> MAEVKANGFPGWLLDPLRPTREKAEPRYRLPEDVRIWAVPLAIGVGLLIVSLVGWAIDARQFYFSYLVGWTFCLTLALGSLFFVMIQHLTRAQWV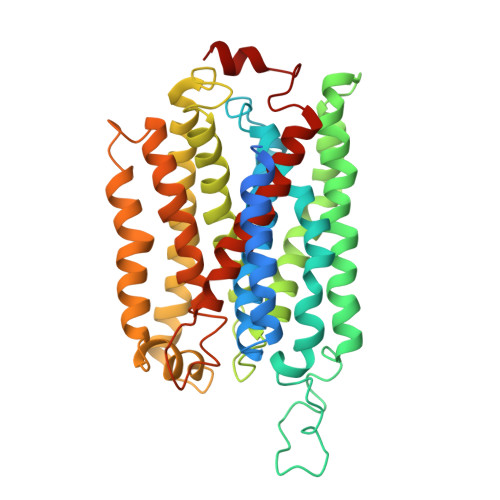VAVRRLPEALVWTFPVLIVLFIPILFGLHDLYHWTHHELYDPSSPEYDPILAGKHAYLNVPFFLVRIAFYFFIWTLLAYKLYTLSVRQDVDPDPSIPAQQRKVSAWGMPLYGVTVAFASYDFLMSLDPHWYSTIFGVYFFAGSFFVALGFITTCYAILVRRGTLQGIVRAPHFQDLGKLMFGFTAFWAYIAFSQYMLIWYGNLPEETLWYRHRLEHGWEVLSQVLIWGHFVLPFLILLPWAAKRTPVLVGTMGIWFAIIHWIDLFWVAMPVLHTEHMTFHWLDVTCWLGLFGVVVGLFFYRISRHSLVPQNDPYLARSLALH>[2x]LDGDQMISHRELWAKIANSINDINEYLKVYEHAVSSYTQMYQDFSAVLSSLAGWISPGGNDGNSVKLQVNSLKKALEELKEKYKDKPLYPANNTVSQEQANKWLTELGGTIGKVSQKNGGYVVSINMTPIDNMLKSLDNLGGNGEVVLDNAKYQAWNAGFSAEDETMKNNLQTLVQKYSNANSIFDNLVKVLSSTISS

Like many Gram-negative pathogens, Shigella rely on their type three secretion system (T3SS) to inject effector proteins into eukaryotic host cells, driving both cellular invasion and evasion of host immune responses. Studies in Shigella have demonstrated that bile salts found in the small intestine (e.g., deoxycholate (DOC)) interact directly with the injectisome tip complex protein invasion plasmid antigen D (IpaD) to support interaction with the hydrophobic translocator protein IpaB and its stable recruitment to the maturing tip complex. In Shigella, IpaD resides at the extracellular tip of the injectisome where it functions as a “gatekeeper” that prevents unwanted protein secretion (leakage) through the injectisome prior to requisite activation events. Here, we uncover critical mechanistic details of the Shigella-specific DOC signaling process by describing the role of a π-helix secondary structure element within the T3SS tip protein invasion plasmid antigen D (IpaD).

X-ray crystal structures of DOC-bound IpaDWT and DOC-bound IpaDΔQ148 were critical for resolving this apparent conflict by providing the first molecular insight into the role of IpaD’s π-helix in the DOC-mediated Shigella virulence enhancement pathway. More specifically, comparing these structures shows that eliminating the π-helix does not eliminate DOC binding, but instead causes the single binding site for DOC to migrate approximately 10 Å, now docking in the cleft between the two central helices where the elimination of the π-helix occurred. A single DOC molecule is also located between the same central helices of IpaD Δ1–121, ΔQ148; however, the binding location of the DOC moved distally nearly 10 Å compared to the IpaDWT binding site, now interacting with the region of the protein where the π-helix once was. A closer look at the side chains located within 4.5 Å of the bound DOCs shows that while some polar and charged side chains such as lysine 137 and serine 141 in the native binding site and aspartate 144 and serine 141 in the modified site of the π-helix deletion construct are in the vicinity of the DOC binding sites, they are oriented away from the bound DOC and do not appear to contribute to binding through electrostatic interactions. Instead, both DOC interactions are driven nearly exclusively through hydrophobic interactions. We first looked within the native (lower) DOC binding site for structural clues as to why it migrated with the elimination of the π-helix and found that the deletion of the π-helix results in a subtle, but noticeable, 15° rotation of the N-terminal helix away from the C-terminal helix. This rotation likely reduces the affinity of DOC to this site as several hydrophobic side chains previously shown to support DOC binding are included in the rotation, but understanding the observed binding site migration also requires consideration of the alternate (distal) binding site that is formed with the loss of the π-helix.>[2x]SSKEVAELKKQVESAELKNQRLKEVFQTKIQEFRKACYTLTGYQIDITTENQYRLTSLYAEHPGDCLIF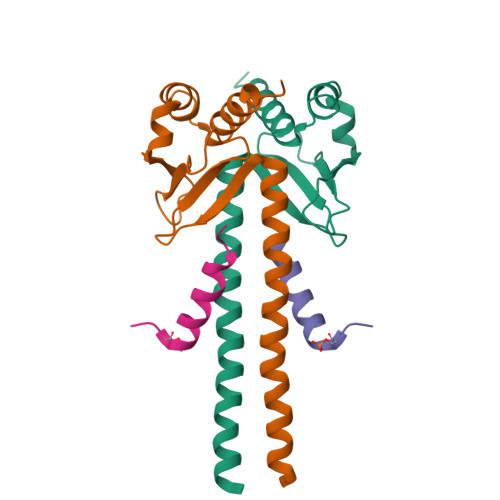KATSPSGSKMQLLETEFSHTVGELIEVHLRRQDSIPAFLSSLTLELFSRQTVA;>[2x]KVQPSPTVHTKEALGFIMNMFQAPTS> AEQSSSEIKIVRDEYGMPHIYANDTWHLFYGYGYVVAQDRLFQMEMARRSTQGTVAEVLGKDFVKFDKDIRRNYWPDAIRAQIAAL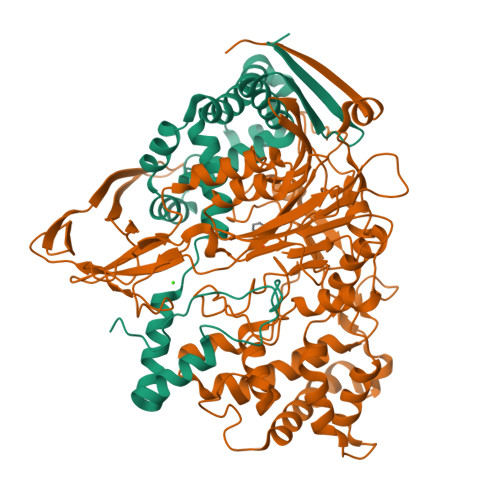SPEDMSILQGYADGMNAWIDKVNTNPETLLPKQFNTFGFTPKRWEPFDVAMIFVGTMANRFSDSTSEIDNLALLTALKDKYGVSQGMAVFNQLKWLVNPSAPTTIAVQESNYPLKFNQQNSQT;> SNMWVIGKSKAQDAKAIMVNGPQFGWYAPAYTYGIGLHGAGYDVTGNTPFAYPGLVFGHNGVISWGSTAGFGDDVDIFAERLSAEKPGYYLHNGKWVKMLSREETITVKNGQAETFTVWRTVHGNILQTDQTTQTAYAKSRAWDGKEVASLLAWTHQMKAKNWQEWTQQAAKQALTINWYYADVNGNIGYVHTGAYPDRQSGHDPRLPVPGTGKWDWKGLLPFEMNPKVYNPQSGYIANWNNSPQKDYPASDLFAFLWGGADRVTEIDRLLEQKPRLTADQAWDVIRQTSRQDLNLRLFLPTLQAATSGLTQSDPRRQLVETLTRWDGINLLNDDGKTWQQPGSAILNVWLTSMLKRTVVAAVPMPFDKWYSASGYETTQDGPTGSLNISVGAKILYEAVQGDKSPIPQAVDLFAGKPQQEVVLAALEDTWETLSKRYGNNVSNWKTPAMALTFRANNFFGVPQAAAEETRHQAEYQNRGTENDMIVFSPTTSDRPVLAWDVVAPGQSGFIAPDGTVDKHYEDQLKMYENFGRKSLWLTKQDVEAHKESQEVLHVQR(1R)-1-(2-chlorophenyl)-2,2,2-tris(fluoranyl)ethanol 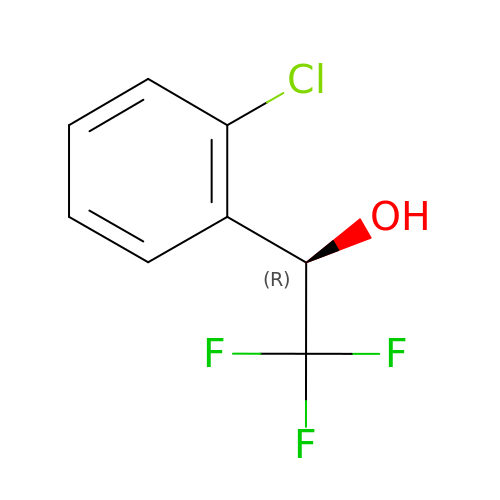| C8 H6 Cl F3 O | HCCWDTPILJKWCQ-SSDOTTSWSA-N3-METHYL-3H-PURIN-6-YLAMINE 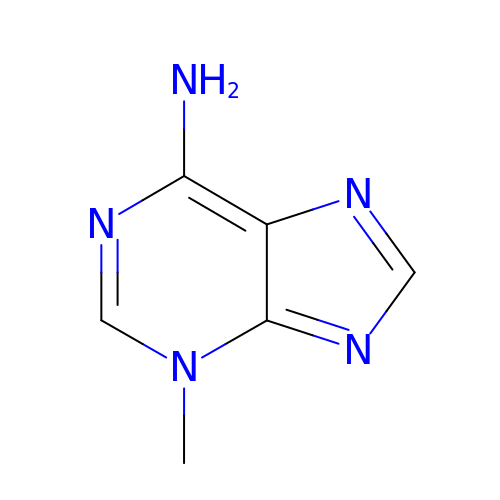| C6 H7 N5 | FSASIHFSFGAIJM-UHFFFAOYSA-N>[13x]MAEKRTGLAEDGAKSVYERLKNDRAPYETRAQNCAQYTIPSLFPKDSDNASTDYQTPWQAVGARGLNNLASKLMLALFPMQTWMRLTISEYEAKQLLSDPDGLAKVDEGLSMVERIIMNYIESNSYRVTLFEALKQLVVAGNVLLYLPEPEGSNYNPMKLYRLSSYVVQRDAFGNVLQMVTRDQIAFGALPEDIRKAVEGQGGEKKADETIDVYTHIYLDEDSGEYLRYEEVEGMEVQGSDGTYPKEACPYIPIRMVRLDGESYGRSYIEEYLGDLRSLENLQEAIVKMSMISSKVIGLVNPAGITQPRRLTKAQTGDFVTGRPEDISFLQLEKQADFTVAKAVSDAIEARLSFAFMLNSAVQRTGERVTAEEIRYVASELEDTLGGVYSILSQELQLPLVRVLLKQLQATQQIPELPKEAVEPTIS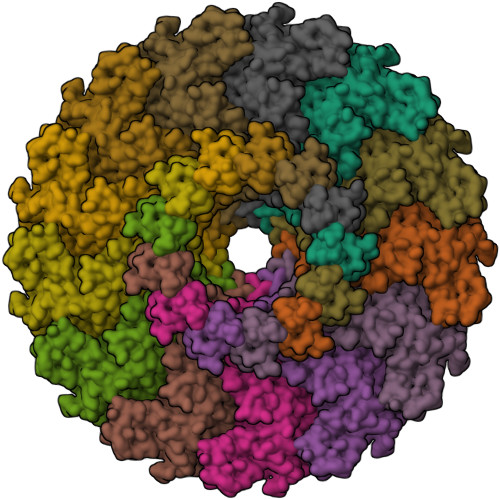TGLEAIGRGQDLDKLERCVTAWAALAPMRDDPDINLAMIKLRIANAIGIDTSGILLTEEQKQQKMAQQSMQMGMDNGAAALAQGMAAQATASPEAMAAAADSVGLQPGIAAALEHHHHHH>AGVFNLEGFGPVSRAMGGTGAAFDIGPAAMMENPATLGLMGEGRHFSLGLDVVSTDIKVTNTATGETASSGNHGNNNGPYFAPQTAFVYRQGRYAFGAGIFAEGGLGTQYGGSSFLSRTSNGVDTGLDQFSRLLVLRVPFSAAYHVTDKLTVGASVDAVWTSLNLGTLLDVSQIGTLAGQGRVSGTLVPTLLGVPGLSGGYIDFSRNAPVGGGVQAWGIGGRLGLTYQVTPDTRIGAAYQAKTHVGDLTGQATLSAVSSVAGNIPLKGDVTVRNFQMPAQLTVGISHQFNDQLSVSADYQRVFWSS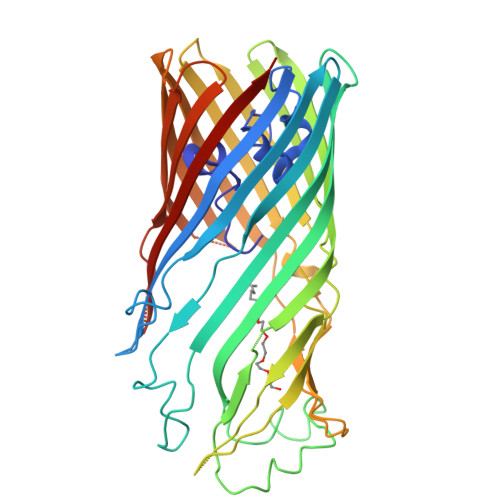VMKDMNVGFVQSGSAANLDLSLPQNYRDISVFGIGAEYRYNAKWTFRGGFHYAQEAIPGNMLLAVVPATPTTSLTGGVSYAIGKNDVIDFALSVALRKTLDNASQPNTAVPISVTHSQVNAVIAYQKRFHHHHHH[2x]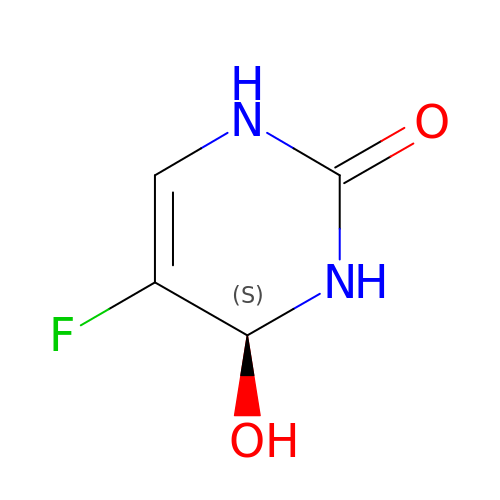(4S)-5-FLUORO-4-HYDROXY-3,4-DIHYDROPYRIMIDIN-2(1H)-ONE | C4 H5 F N2 O2 | PRVUBDAKZJCBTI-VKHMYHEASA-N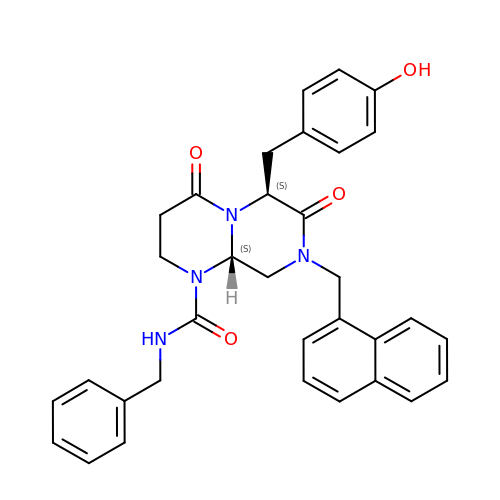(5R,6S,9aS)-N-benzyl-6-[(4-hydroxyphenyl)methyl]-8-[(naphthalen-1-yl)methyl]-4,7-dioxohexahydro-2H-pyrazino[1,2-a]pyrimidine-1(6H)-carboxamide | C33 H32 N4 O4 | HQWTUOLCGKIECB-XZWHSSHBSA-N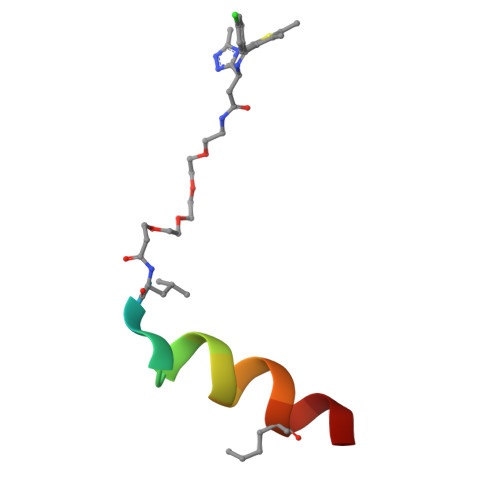> XXLTFXEYWAQLLSAA> ELNPNAEVWGAPV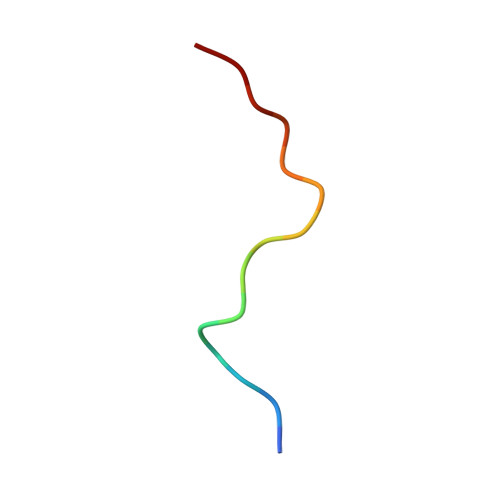LH>MDYKDDDDKGTDYKDDDDKSGSLEVLFQGPMSLVLNDLLICCRQLEHDRATERKKEVEKFKRLIRDPETIKHLDRHSDSKQGKYLNWDAVFRFLQKYIQKETECLRIAKPNVSASTQASRQKKMQEISSLVKYFIKCANRRAPRLKCQELLNYIMDTVKDSSNGAIYGADCSNILLKDILSVRKYWCEISQQQWLELFSVYFRLYLKPSQDVHRVLVARIIHAVTKGCCSQTDGLNSKFLDFFSKAIQCARQEKSSSGLNHILAALTIFLKTLAVNFRIRVCELGDEILPTLLYIWTQHRLNDSLKEVIIELFQLQIYIHHPKGAKTQEKGAYESTKWRSILYNLYDLLVNEISHIGSRGKYSSGFRNIAVKENLIELMADICHQVFNEDTRSLEISQSYTTTQRESSDYSVPCKRKKIELGWEVIKDHLQKSQNDFDLVPWLQIATQLISKYPASLPNCELSPLLMILSQLLPQQRHGERTPYVLRCLTEVALCQDKRSNLESSQKSDLLKLWNKIWCITFRGISSEQIQAENFGLLGAIIQGSLVEVDREFWKLFTGSACRPSCPAVCCLTLALTTSIVPGTVKMGIEQNMCEVNRSFSLKESIMKWLLFYQLEGDLENSTEVPPILHSNFPHLVLEKILVSLTMKNCKAAMNFFQSVPECEHHQKDKEELSFSEVEELFLQTTFDKMDFLTIVRECGIEKHQSSIGFSVHQNLKESLDRCLLGLSEQLLNNYSSEITNSETLVRCSRLLVGVLGCYCYMGVIAEEEAYKSELFQKAKSLMQCAGESITLFKNKTNEEFRIGSLRNMMQLCTRCLSNCTKKSPNKIASGFFLRLLTSKLMNDIADICKSLASFIKKPFDRGEVESMEDDTNGNLMEVEDQSSMNLFNDYPDSSVSDANEPGESQSTIGAINPLAEEYLSKQDLLFLDMLKFLCLCVTTAQTNTVSFRAADIRRKLLMLIDSSTLEPTKSLHLHMYLMLLKELPGEEYPLPMEDVLELLKPLSNVCSLYRRDQDVCKTILNHVLHVVKNLGQSNMDSENTRDAQGQFLTVIGAFWHLTKERKYIFSVRMALVNCLKTLLEADPYSKWAILNVMGKDFPVNEVFTQFLADNHHQVRMLAAESINRLFQDTKGDSSRLLKALPLKLQQTAFENAYLKAQEGMREMSHSAENPETLDEIYNRKSVLLTLIAVVLSCSPICEKQALFALCKSVKENGLEPHLVKKVLEKVSETFGYRRLEDFMASHLDYLVLEWLNLQDTEYNLSSFPFILLNYTNIEDFYRSCYKVLIPHLVIRSHFDEVKSIANQIQEDWKSLLTDCFPKILVNILPYFAYEGTRDSGMAQQRETATKVYDMLKSENLLGKQIDHLFISNLPEIVVELLMTLHEPANSSASQSTDLCDFSGDLDPAPNPPHFPSHVIKATFAYISNCHKTKLKSILEILSKSPDSYQKILLAICEQAAETNNVYKKHRILKIYHLFVSLLLKDIKSGLGGAWAFVLRDVIYTLIHYINQRPSCIMDVSLRSFSLCCDLLSQVCQTAVTYCKDALENHLHVIVGTLIPLVYEQVEVQKQVLDLLKYLVIDNKDNENLYITIKLLDPFPDHVVFKDLRITQQKIKYSRGPFSLLEEINHFLSVSVYDALPLTRLEGLKDLRRQLELHKDQMVDIMRASQDNPQDGIMVKLVVNLLQLSKMAINHTGEKEVLEAVGSCLGEVGPIDFSTIAIQHSKDASYTKALKLFEDKELQWTFIMLTYLNNTLVEDCVKVRSAAVTCLKNILATKTGHSFWEIYKMTTDPMLAYLQPFRTSRKKFLEVPRFDKENPFEGLDDINLWIPLSENHDIWIKTLTCAFLDSGGTKCEILQLLKPMCEVKTDFCQTVLPYLIHDILLQDTNESWRNLLSTHVQGFFTSCLRHFSQTSRSTTPANLDSESEHFFRCCLDKKSQRTMLAVVDYMRRQKRPSSGTIFNDAFWLDLNYLEVAKVAQSCAAHFTALLYAEIYADKKSMDDQEKRSLAFEEGSQSTTISSLSEKSKEETGISLQDLLLEIYRSIGEPDSLYGCGGGKMLQPITRLRTYEHEAMWGKALVTYDLETAIPSSTRQAGIIQALQNLGLCHILSVYLKGLDYENKDWCPELEELHYQAAWRNMQWDHCTSVSKEVEGTSYHESLYNALQSLRDREFSTFYESLKYARVKEVEEMCKRSLESVYSLYPTLSRLQAIGELESIGELFSRSVTHRQLSEVYIKWQKHSQLLKDSDFSFQEPIMALRTVILEILMEKEMDNSQRECIKDILTKHLVELSILARTFKNTQLPERAIFQIKQYNSVSCGVSEWQLEEAQVFWAKKEQSLALSILKQMIKKLDASCAANNPSLKLTYTECLRVCGNWLAETCLENPAVIMQTYLEKAVEVAGNYDGESSDELRNGKMKAFLSLARFSDTQYQRIENYMKSSEFENKQALLKRAKEEVGLLREHKIQTNRYTVKVQRELELDELALRALKEDRKRFLCKAVENYINCLLSGEEHDMWVFRLCSLWLENSGVSEVNGMMKRDGMKIPTYKFLPLMYQLAARMGTKMMGGLGFHEVLNNLISRISMDHPHHTLFIILALANANRDEFLTKPEVARRSRITKNVPKQSSQLDEDRTEAANRIICTIRSRRPQMVRSVEALCDAYIILANLDATQWKTQRKGINIPADQPITKLKNLEDVVVPTMEIKVDHTGEYGNLVTIQSFKAEFRLAGGVNLPKIIDCVGSDGKERRQLVKGRDDLRQDAVMQQVFQMCNTLLQRNTETRKRKLTICTYKVVPLSQRSGVLEWCTGTVPIGEFLVNNEDGAHKRYRPNDFSAFQCQKKMMEVQKKSFEEKYEVFMDVCQNFQPVFRYFCMEKFLDPAIWFEKRLAYTRSVATSSIVGYILGLGDRHVQNILINEQSAELVHIDLGVAFEQGKILPTPETVPFRLTRDIVDGMGITGVEGVFRRCCEKTMEVMRNSQETLLTIVEVLLYDPLFDWTMNPLKALYLQQRPEDETELHPTLNADDQECKRNLSDIDQSFNKVAERVLMRLQEKLKGVEEGTVLSV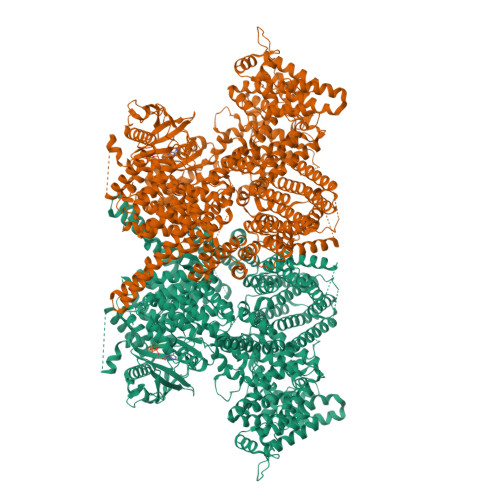GGQVNLLIQQAIDPKNLSRLFPGWKAWV[2x]>MAFTNYSSLNRAQLTFEYLHTNSTTHEFLFGALAELVDNARDADATRIDIYAERREDLRGGFMLCFLDDGAGMDPSDAASVIQFGKSAKRTPESTQIGQYGNGLKSGSMRIGKDFILFTKKEDTMTCLFLSRTFHEEEGIDEVIVPLPTWNARTREPVTDNVEKFAIETELIYKYSPFRTEEEVMTQFMKIPGDSGTLVIIFNLKLMDNGEPELDIISNPRDIQMAETSPEGTKPERRSFRAYAAVLYIDPRMRIFIHGHKVQTKRLSCCLYKPRMYKYTSSRFKTRAEQEVKKAEHVARIAEEKAREAESKARTLEVRLGGDLTRDSRVMLRQVQNRAITLRREADVKKRIKEAKQRALKEPKELNFVFGVNIEHRDLDGMFIYNCSRLIKMYEKVGPQLEGGMACGGVVGVVDVPYLVLEPTHNKQDFADAKEYRHLLRAMGEHLAQYWKDIAIAQRGIIKFWDEFGYLSANWNQPPSSELRYKRRRAMEIPTTIQCDLCLKWRTLPFQLSSVEKDYPDTWVCSMNPDPEQDRCEASEQKQKVPLGTFRKDMKTQEEKQKQLTEKIRQQQEKLEALQKTTPIRSQADLKKLPLEVTTRPSTEEPVRRPQRPRSPPLPAVIRNAPSRPPSLPTPRPASQPRKAPVISSTPKLPALAAREEASTSRLLQPPEAPRKPANTLVKTASRPAPLVQQLSPSLLPNSKSPREVPSPKVIKTPVVKKTEAPIKLAPATPSRKRAVAVADEEEVEEEAERRKERCKRGRFVVKEEKKDSNELADAAGEEDSADLKRAQKDKGLHVEVRVNREWYTGRVTAVEVGKHVVRWKVKFDYVPTDTTPRDRWVEKGSEDVRLMKPPSPEHQSLDTQQEGGEEEVGPVAQQAIAVAEPSTSECLRIEPDTTALSTNHETIDLLVQILRNCLRYFLPPSFPISKKQLSAMNSDELISFPLKEYFKQYEVGLQNLCNSYQSRADSRAKASEESLRTSERKLRETEEKLQKLRTNIVALLQKVQEDIDINTDDELDAYIEDLITKGD[2x]

The Microrchidia (MORC) family of chromatin-remodelling ATPases is pivotal in forming higher-order chromatin structures that suppress transcription. All MORCs share three features: an N-terminal gyrase, heat shock protein 90, histidine kinase and MutL (GHKL) ATPase domain, a central CW-type zinc finger (CW) domain, and a divergent C-terminal domain (CTD) with predicted coiled coils (CCs). MORC2 possesses multiple DNA-binding sites that undergo structural rearrangement upon DNA binding. Importantly, MORC2 mediates chromatin remodelling via ATP hydrolysis-dependent DNA compaction in vitro, regulated by the phosphorylation state of its CTD.

To determine how phosphorylation of MORC2 affects DNA binding, we purified a MORC2 phosphodead (MORC2PD) mutant comprising S725A, S730A, S739A, S743A, S777A and S779A mutations. We determined the structures of MORC2PD and MORC2 ATPase domain with (MORC2PD-DNA, MORC21-603-DNA) and without DNA (MORC2PD, MORC21-603), in presence of AMP-PNP, at overall resolutions of 1.9, 2.5, 2.4 and 3.2 Å, respectively, using cryoEM. Although there were 2D classes where MORC2 was bound to the DNA in the MORC2PD-DNA samples, these could not be resolved into a 3D structure due to low resolution and absence of diverse views, suggesting that there may be an increase in flexibility upon DNA binding despite similar global resolution observed in DNA or DNA-free samples. Interestingly, almost all CC1 was missing in the DNA-bound cryoEM structures indicating high flexibility of this region upon DNA binding. The dimerised ATPase domain is well-resolved in all the cryoEM maps, but no density is seen for CTD to model in the full-length MORC2PD, MORC2PD-DNA and MORC2S87A maps. MORC2 constructs containing either phosphorylated or non-phosphorylated CTDs did not induce large structural changes in the ATPase domain upon DNA binding, revealing that the ATPase core is highly stable in the presence of AMP-PNP. The observed flexibility of CC1 inferred from its absence in the DNA-bound MORC2 cryoEM structures and crosslinking mass spectrometry, suggests that CC1 may aid in binding and compacting DNA. The ability of MORC2 to bind DNA through its multiple sites, combined with the flexibility of its CTD relative to the ATPase domain, explains why it is hard to determine DNA-bound MORC2 structures.> SMMSDLHIPGTQSTPAIQGDWQAGRLSMQGDSYPENSYELFGQVIDWVERFLADGQRPLELDLRLLYLNTSSIKAMMDILDLLEEAHQGGRPVSLRWHYDR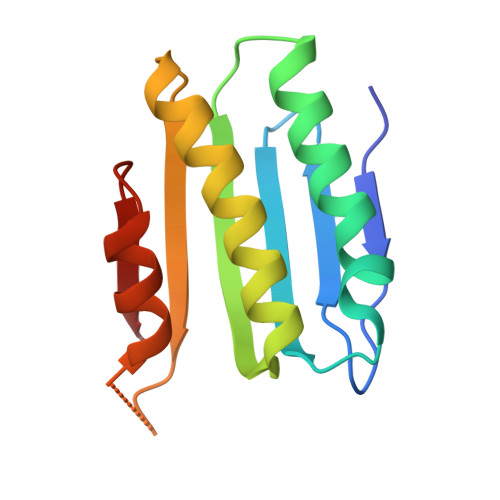RNERVAELAEEFREDCSFPFAIQAHDE> GKKKVRKYWD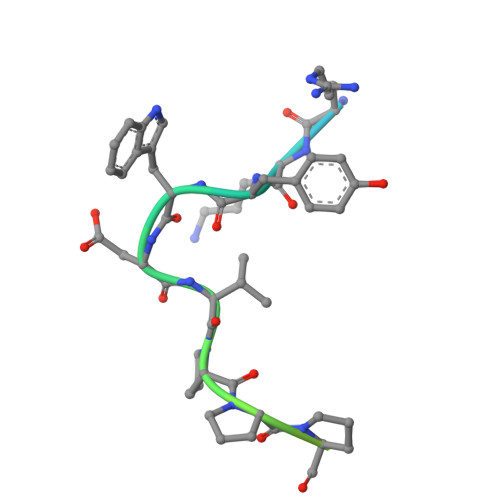VPPPGFEHITPMQYKAMQA Leukotriene (LT) C4 synthase (LTC4S) catalyzes the conjugation of the fatty acid LTA4 with the tripeptide GSH to produce LTC4, the parent compound of the cysteinyl leukotrienes, important mediators of asthma. LTC4S is a trimeric integral membrane protein and a member of the MAPEG (membrane-associated proteins in eicosanoid and glutathione metabolism) family, which also includes three microsomal GSH S-transferases, 5-lipoxygenase activating protein, and microsomal prostaglandin E synthase 1 (9, 10). The crystal structure of human LTC4S has been solved and identified a unique horseshoe-shaped conformation of GSH bound at the active site by residues from two neighboring monomers. It was postulated that the lipid substrate LTA4 binds in a hydrophobic crevice between two monomers and that Trp-116 could act as a “molecular ruler” for binding of LTA4 with its ω-end buried under the aromatic side chain.

We exchanged Trp-116 in LTC4S for an Ala or Phe residue and analyzed the effects on catalysis and kinetic parameters. To further probe the role of Trp-116 for the positioning of LTA4 at the active site, we solved the structures of W116A and W116F LTC4S in complex with analog I, at 2.7 and 2.4 Å resolution, respectively. Of special note, in the structure of the mutant W116F, the phenyl ring has adopted a tilted conformation due to rotation at the α-β and β-γ carbon bonds. This rotamer opens the protein cavity toward the lipid bilayer. In the W116F mutant, the phenylalanine is now pointing outwards to the solution/lipid bilayer and no longer functions as a “lid” for the hydrophobic pocket as seen with the Trp-116 in the WT structure. Considering the inherent variability that comes with enzyme assays with highly unstable lipid substrates, no major kinetic alterations were observed, thus demonstrating that Trp-116 is not essential for catalysis. The 3-fold increased LTA4 turnover of the W116F mutant may reflect a Phe configuration, which leaves the active site open to the lipid bilayer, thus facilitating product release (see below). To detail binding interactions and analog positions, we used the structures of LTC4S and the mutant W116F in complex with analog I because they have the best interpretable electron densities. The sulfur in analog I in the W116A and W116F mutants shows a larger shift of ∼7.1 Å. In the W116A and W116F mutants, the three terminal carbons shift by ∼3.5 Å upwards toward the position of the Trp-116. This is most likely due to the larger space available in the absence of the tryptophan residue.

> MHHHHHHKDEVALLAAVTLLGVLLQAYFSLQVISARRAFRVSPPLTTGPPEFERVYRAQVNCSEYFPLFLATLWVAGIFFHEGAAALCGLVYLFARLRYFQGYARSAQLRLAPLYASARALFLLVALAALGLLAHFLPAALRAALLGRLRTLLPWA> GRPRPEVAHQLFRCFQYQEDMGPRASLGRLRELCNHWLRPALHTKKQILELLVLEQFLSVLPPH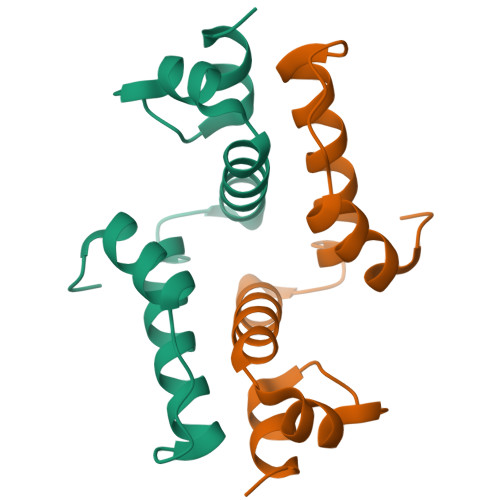VLSRLHGAPLRDGEEVAQLEGVPRDISHM>ASNQVTLAFANDAEISAFGFCTASEAVSYYSEAAASGFMQCRFVSFDLADTVEGLLPEDYVMVVVGTTKLSA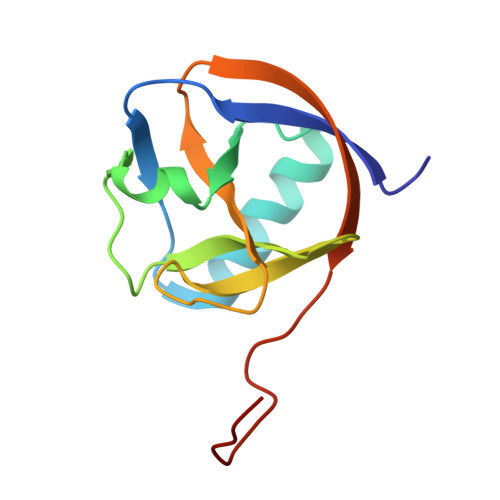YVDTFGSRPRNICGWLLFSNCNYFLEELELTFGRRGGLEHHHHHHH[2x]>[4x]MERKHHFVLVHNAYHGAWIWYKLKPLLESAGHRVTAVELAASGIDPRPIQAVETVDEYSKPLIETLKSLPENEEVILVGFSFGGINIALAADIFPAKIKVLVFLNAFLPDTTHVPSHVLDKYMEMPGGLGDCEFSSHETRNGTMSLLKMGPKFMKARLYQNCPIEDYELAKMLHRQGSFFTEDLSKKEKFSEEGYGSVQRVYVMSSEDKAIPCDFIRWMIDNFNVSKVYEIDGGDHMVMLSKPQKLFDSLSAIATDYM

Hydroxynitrile lyases (HNLs) catalyze the cleavage of cyanohydrins into the corresponding carbonyl compound and hydrocyanic acid. In 2007 a hydroxynitrile lyase from the noncyanogenic plant Arabidopsis thaliana (mouse-ear cress) was discovered (AtHNL) which exhibits high sequence similarity to the S-selective HbHNL (45 % identity and 67 % similarity) but quite unexpectedly was found to be R-selective for a wide range of converted cyanohydrins. Previously, S selectivity has been considered a characteristic feature of HNLs from the α/β-hydrolase family, and AtHNL is thus the first R-selective member of this fold family. The Ser-His-Asp catalytic triad is conserved in AtHNL and is crucial for catalysis, whereas HbHNL and AtHNL differ with respect to several other residues surrounding the active site.

The crystal structure of AtHNL shows a striking structural similarity between AtHNL and HbHNL, both in the polypeptide fold and with respect to the presence and location of crucial active site residues, for example, the Ser-His-Asp catalytic triad. The only significant fold difference between the two structures is observed in a loop at the entrance of the active site. The asymmetric unit consists of four protein molecules forming two independent dimers. Contacts between the two protein chains are mostly hydrophobic in nature but also include a salt-bridge interaction between Lys24 of one molecule and Glu165 of the other. The PISA-analysis on the interaction surfaces indicates that the dimeric arrangement is also likely to be present in solution. Specifically, the lysine residue crucial for stabilizing the negative charge on the cyanide (Lys236 in HbHNL) is replaced by methionine. In the modeled complex with (R)-mandelonitrile the hydroxyl group of the substrate is hydrogen bonded to His236, and also interacts with the amide group of Asn12. The cyano group is oriented toward the main-chain NH-groups of Phe82 and Ala13 and is located at the N-terminal end of the α-helix following the “nucleophile elbow” in the α/β-hydrolase fold. While the R enantiomer has the hydroxyl group within hydrogen bonding distance to a potential catalytic base (His236), the S enantiomer interacts with a main-chain carbonyl oxygen, which is unlikely to deprotonate a hydroxyl group. In contrast to HbHNL (and MeHNL), however, the latter is not accomplished by a positively charged (lysine) residue but presumably by a combination of main-chain amide hydrogen bonds and a helix dipole more similar to the stabilization of the oxyanion in α/β-hydrolases.>MALKSLVLLSLLVLVLLLVRVQPSLGKETAAAKFERQHMDSSTSAASSSNYCNQMMKSRNLTKDRCKPVNTFVHESLADVQAVCSQKNVACKNGQTNCYQSYSTMSITDCRETGSSKYPN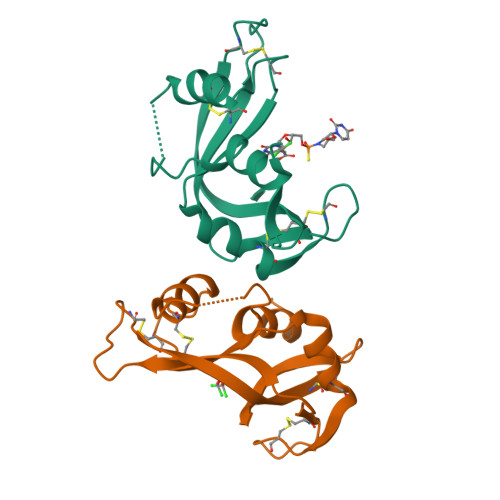CAYKTTQANKHIIVACEGNPYVPVHFDASV[2x]>MGSSHHHHHHSQDPNSMSAVQPFIRTNIGSTLRIIEEPQRDVYWIHMHADLAINPGRACFSTRLVDDITGYQTNLGQRLNTAGVLAPHVVLASDSDVFNLGGDLALFCQLIREGDRARLLDYAQRCVRGVHAFHVGLGARAHSIALVQGN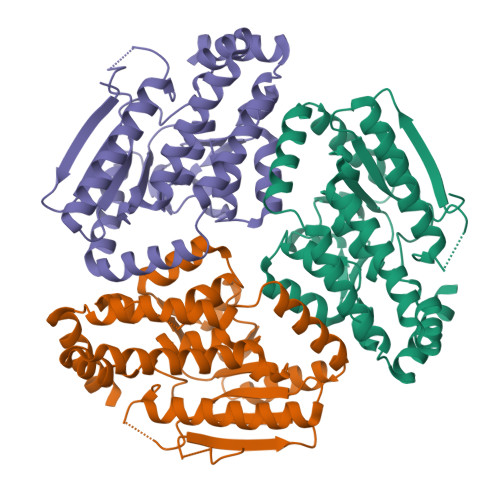ALGGGFEAALSCHTIIAEEGVMMGLPEVLFDLFPGMGAYSFMCQRISAHLAQKIMLEGNLYSAEQLLGMGLVDRVVPRGQGVAAVEQVIRESKRTPHAWAAMQQVREMTTAVPLEEMMRITEIWVDTAMQLGEKSLRTMDRLVRAQSRRSGLDAG[3x]> RRGALIVLEGVDRAGKSTQSRKLVEALCAA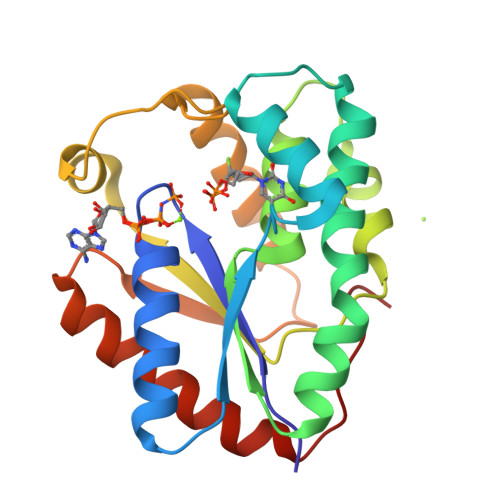GHRAELLRFPERSTEIGKLLSSYLQKKSDVEDHSVHLLFSANRWEQVPLIKEKLSQGVTLVVDRYAFSGVAFTGAKENFSLDWCKQPDVGLPKPDLVLFLQLQLADAAKRGAFGHERYENGAFQERALRCFHQLMKDTTLNWKMVDASKSIEAVHEDIRVLSEDAIATATEKPLGELWK>[8x]MKVNKKRLAEIFNVDPRTI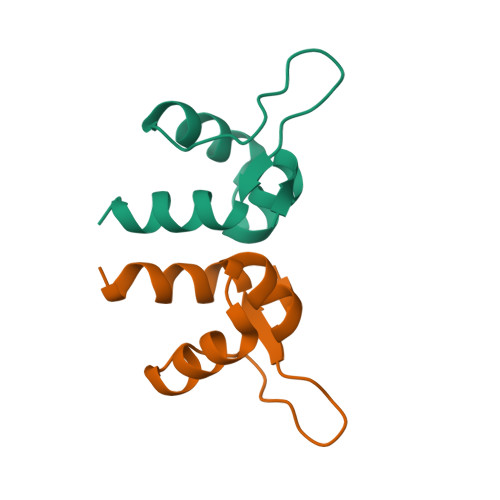ERWQSQGLPCASKGSKGIESVFDTAMAIQWYAQRE>LTGQIIEYTIKIQTIYTGNFKHKNGFLKMIERGIAMKKENLKILAKKAQTIAIVGANYRFATRVLLENLDKMDFTGTIYLVNPRYENIDGVRCYQSLLEIEDTIDVVVGLVNPQLMIQVASNASKINAKVLVIPGGGYGESGVEGQNIQNAILERAADSGMRIVGPNCMGYLNMHAQFTPYIGTLHRPLRPIKKGPVSIISQSGSVNDAFIASKLGISKIYSTGNEADVQMHDYLNLLAEDPETSVIILYIEAIRNHLSFLRALDLCSKNKKPVIAIKVGRTIKSAAVANAHSGALAGDYEIEKLFLEGHGVLFVEDIDQAVAVALLLSQPYLPTVNTVAALTVSGGQAGILLDLAEDYGVDFPDFSAVTNYEIASKLPELGGLSNPLDIWGKSSKDFSEVSNICLSSIVKDADIGIITVAIDAPIGQGDHEFDFTSIPAKDLASLRGNSDKPFLYFSHIQTEFDPRVESILDEAGIAVIQGSRNALVACRALFKYKEFLEKNNHTPIYSVEDLSIQKGLKLLHDNEGRKLLDESGFVSPREQVVTSLQEGVDYAESIGYPVVLKAQGLAHKTDVGGVALNIKSAAKLKKAWGKMEHLNSPYYLIQEMVTDGFETILAYRTDMNYGPVVIFGLGGIYTELFNEVVLAVPPITHKKAEQMVKSIPMLWKSIEGYRGNPALDLEALTASIVQMGETAMEKYEEIVEFEINPLSVRVKGVVALDVLASVKTTAAKEADAEEADVKKCSELV[4x]

Genetic and biochemical work showed that Psychrobacter sp. D2 possesses a novel DMSP lyase termed DddX for DMSP catabolism. DddX is an ATP-dependent DMSP lyase which catalyzes a two-step reaction: the ligation of DMSP and CoA, and the cleavage of DMSP-CoA to produce DMS and acryloyl-CoA. Sequence analysis suggests that DddX is an acetate-CoA ligase, which belongs to the acyl-CoA synthetase (ACD) superfamily and requires CoA and ATP as co-substrates for catalysis. Diverse DMSP lyases in some algae, bacteria, and fungi cleave DMSP to yield gaseous dimethyl sulfide (DMS), an infochemical with important roles in atmospheric chemistry.

To elucidate the structural basis of DddX catalysis, we solved the crystal structure of DddX in complex with ATP by the single-wavelength anomalous dispersion method using a selenomethionine derivative (Se-derivative). Although there are four DddX monomers arranged as a tetramer in an asymmetric unit, gel filtration analysis indicated that DddX maintains a dimer in solution. Each DddX monomer contains a CoA-binding domain and an ATP-grasp domain, with one loop (Gly280-Tyr300) of the CoA-binding domain inserting into the ATP-grasp domain. ATP is bound in DddX mainly via hydrophilic interactions, including hydrogen bonds and salt bridges. The overall structure of DddX is similar to that of NDP-forming acetyl-CoA synthetase ACD1 (Weiße et al., 2016), with a root mean square deviation (RMSD) between these two structures of 4.6 Å over 581 Cα atoms. ACD1 consists of separate α- and β-subunits, which corresponds to the CoA-binding domain and the ATP-grasp domain of DddX, respectively. Sequence alignment indicated that His292 of DddX is likely the conserved histidine residue to be phosphorylated, and Gly280-Tyr300 is likely the ‘swinging loop’. In the crystal structure of DddX, His292 from loop Gly280-Tyr300 directly forms a hydrogen bond with the γ-phosphate of ATP, suggesting a potential for phosphorylation, which is further supported by mutational analysis. Mutation of His292 to alanine abolished the activity of DddX, indicating the key role of His292 during catalysis. Firstly, His292 is phosphorylated by ATP, forming phosphohistidine, which will be brought to the CoA-binding domain through the conformational change of the swinging loop Gly280-Tyr300.>MNQTLETGTTTVGITLKDAVIMATERRVTMENFIMHKNGKKLFQIDTYTGMTIAGLVGDAQVLVRYMKAELELYRLQRRVNMPIEAVATLLSNMLNQVKYMPYMVQLLVGGIDTAPHVFSIDAAGGSVEDIYASTGSGSPFVYGVLESQYSEKMTVDEGVDLVIRAISAAKQRDSASGGMIDVAVITRKDGYVQLPTDQIESRIRKLGLIL[14x];>AYDRAITVFSPDGRLFQVEYAREAVKKGSTALGMKFANGVLLISDKKVRSRLIEQNSIEAIQLIDDYVAAVTSGLVADARVLVDFARISAQQEKVTYGSLVNIENLVKRVADQMQQYTQYGGVRPYGVSLIFAGIDQIGPRLFDCDPAGTINEYKATAIGSGKDAVVSFLEREYKENLPEKEAVTLGIKALKSSLEEGEELKAPEIASITVGNKYRIYDQEEVKKFL[7x];>[7x]AYDRAITVFSPDGRLFQVEYALEAVKKGSTALGMKFANGVLLISDKKVRSRLIEQNSIEKIQLIDDYVAAVTSGLVADARVLVDFARISAQQEKVTYGSLVNIENLVKRVADQMQQYTQYGGVRPYGVSLIFAGIDQIGPRLFDCDPAGTINEYKATAIGSGKDAVVSFLEREYKENLPEKEAVTLGIKALKSSLEEGEELKAPEIASITVGNKYRIYDQEEVKKFL

In archaea, the 20S is composed of homo-heptameric α- and β-rings, and PAN (Proteasomal Activator Nucleotidase), a homohexamer proteasomal ATPase, is the RP found in many species. Unfolded substrates enter the chamber through a narrow pore in the center of α-rings, where N-termini of α-subunits form a gate to impede unregulated access to the proteolytic chamber. We designed and assembled in vitro various asymmetric archaea 20S, in which one of the two α-rings contains a point mutation, K66A, which prevents RP binding to the α-ring. Our studies reveal that, upon binding of a RP with a conserved C-terminal HbYX motif to one α-ring, the gate of the opposite α-ring opens allosterically, resulting in similar proteolytic activities of 20S singly capped and doubly capped with PAN.

The first one is a wild-type homo-hexameric PAN ATPase, homologous to the Rpt ATPase subunits in the base of 19S in  eukaryotic 26S proteasomes. The C-terminus of PAN contains an HbYX (hydrophobic, tyrosine, and any amino acid) motif that is required for binding to the α-ring and opening its gate. We also determined structures of PAN-αWTββαK66A in the presence of ATP, without and with substrate GFP-ssrA, both to resolutions of 3.4 Å. Because of the symmetry mismatch between the heptameric α-ring and hexameric PAN ATPase, PAN does not engage with α-ring symmetrically, and not every binding pocket in the CP is occupied by a C-terminus of PAN. To obtain sufficient resolution to evaluate the gate conformation, we applied a C7 symmetry. Thus, the density of PAN in this reconstruction does not represent its correct structure. Even so, the conformation of the gate in the C7 symmetrized density map still represents the state of the gate. Whether without or with the substrate, the proximal gates are in an open conformation, consistent with the gate opening by the C-termini of PAN with its native C-terminal HbYX motif. Furthermore, the C7 symmetry averaged density map still shows rotation of α-subunits induced by binding of PAN’s C-termini. Thus, structures of PA26PANc-αWTββαK66A and PAN-αWTββαK66A both show that the gate of the distal α-ring is open even without direct association with an activator; this distal gate is opened allosterically by the engagement of an activator to the proximal α-ring.>MHKIGETFKAGHTNFTVNKVDRVQKGEYMNVGGAVNEETKTIKDDEERLII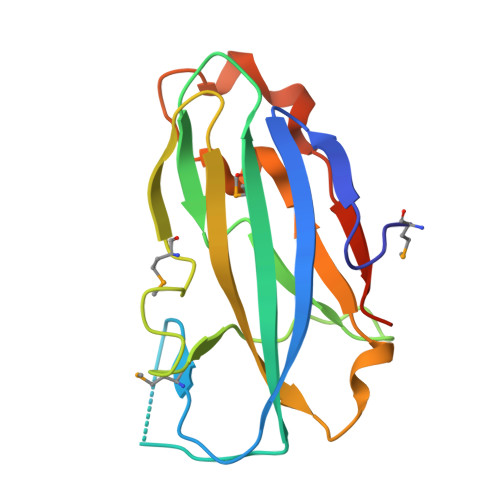EVTMENIGEDSISYNFIGFDLRDKNDQSVRPVFSIEEKGRILMGGTLVSGKKVTGVLSYVIPKGEQKHYTLVYNPFLADTNSSNTEERVKDDIDYLVKLDLEHHHHHH[2x]(5R)-5-{[1-(4-fluorophenyl)-1H-1,2,3-triazol-4-yl]methyl}-5-methylpyrrolidine-2,4-dione 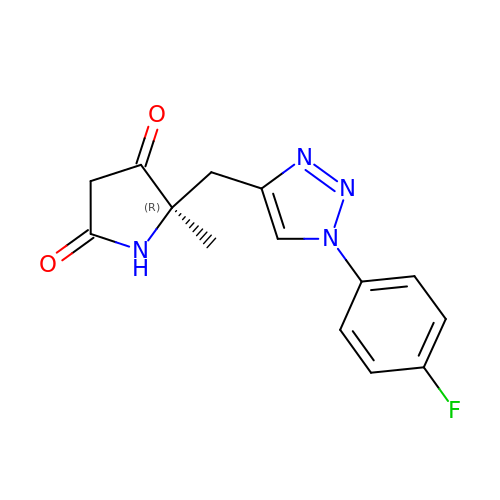| C14 H13 F N4 O2 | UUBOMXRWPFJYHC-CQSZACIVSA-N>[6x]AKLTIESTPFNVAEGKEVLLLAHNLPQNRIGYSWYKGERVDGNSLIVGYVIGTQQATPGPAYSGRETIYPNAS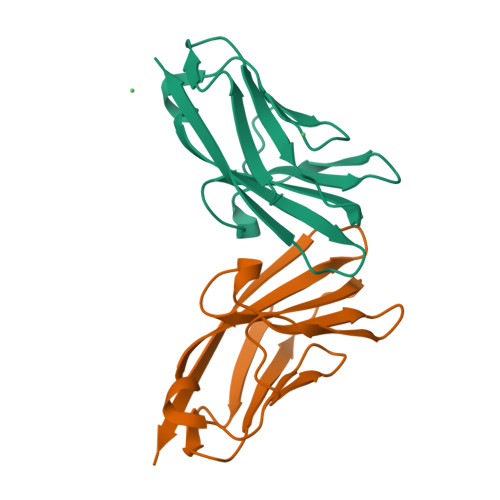LLIQNVTQNDTGFYTLQVIKSDLVNEEATGQFHVY;>[6x]AQLTIEAVPSNAAEGKEVLLLVHNLPQDPRGYNWYKGETVDANRRIIGYVISNQQITPGPAYSNRETIYPNASLLMRNVTRNDTGSYTLQVIKLNLMSEEVTGQFSVHC>PIISEGNRNRHRAWALRELQDIKKEIENKAPGSQVWIQTLRLAILQADPTPADLEQLCQYIASPVDQTAHMTSLTAAIAAAEAANTLQGFNPQNGTLTQQSAQPNAGDLRSQYQNLWLQAWKNLPTRPHHHHH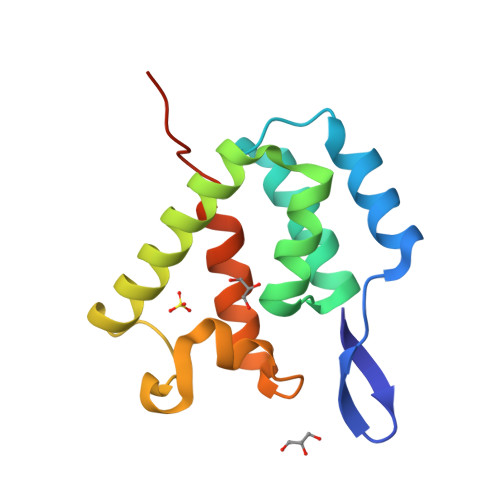H[2x]~{N}-[3-[(5-ethanoyl-2-ethoxy-phenyl)carbamoyl]-5-(1-methylpyrazol-3-yl)phenyl]-5-[(4-methylpiperazin-1-yl)methyl]furan-2-carboxamide 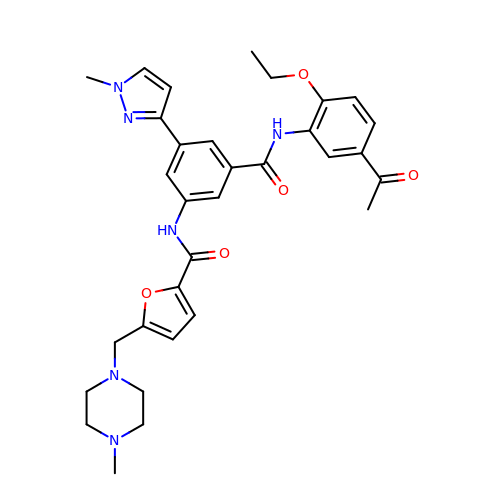| C32 H36 N6 O5 | UOPWJMNPOBVGRX-UHFFFAOYSA-N> TIQNDIPDLYSVFKDYFPIGVAVDPSRLNDADPHAQLTAKHFNMLVAENAMKPESLQPTEGNFTFDNADKIVDYAIAHNMKMRGHTLLWHNQVPDWFFQDPSDPSKPASRDLLLQRLRTHITTVLDHFKTKYGSQNPIIGWDVVNAVLDDNGNLRNSKWLQIIGPDYIEKAFEYAHEADPSMKLFINDYNIENNGVKTQAMYDLVKKLKNEGVPINGIGMQMHISINSNIDNIKASIEKLASLGVEIQVTELDMNMNGDVSNDALLKQAR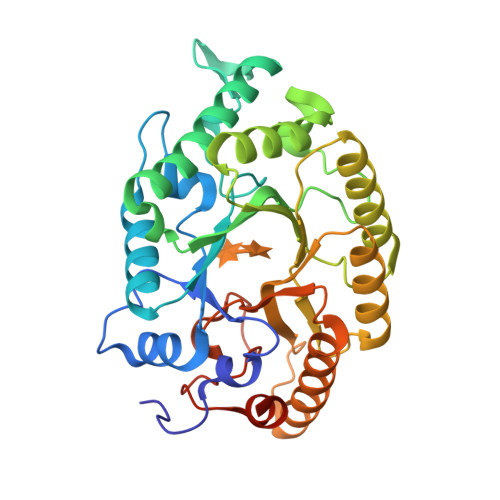LYKQLFDLFKAEKQYITAVVFWGVSDDVSWLSKPNAPLLFDSKLQAKPAYWAIVDLGKAIPDIQSA> DSGE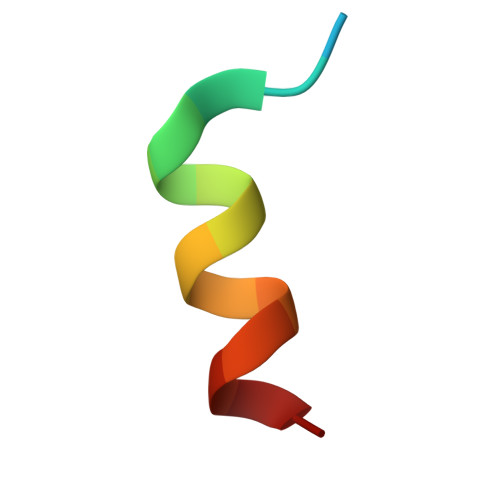SLEDLMAKMKNM>[2x]MNVTVDQSTLAGATRGIVRGGETLKEHRDRLMAATKATGRYAGLKTLELREREPILYNKLFSRLRAGVVDARETAKKIAASPIVEQEGELCFTLYNAAGDSLLTSTGIIIHVGTMGAAIKYMIENNWEANPGVHDKDIFCNNDSLIGNVHPCDIHTIVPIFWEGELIGWVGGVTHVIDTGAVGPGSMATGQVQRFGDGYSITCRKVGANDTLFRDWLHESQRMVRTTRYWMLDERTRIAGCHMIRKLVEEVVAEEGIEAYWKFAYEAVEHGRLGLQARIKAMTIPGTYRQVGFVDVPYAHEDVRVPSDFAKLDTIMHAPCEMTIRRDGTWRLDFEGSSRWGWHTYNAHQVSFTSGIWVMMTQTLIPSEMINDGAAYGTEFRLPKGTWMNPDDRRVAFSYSWHFLVSAWTALWRGLSRSYFGRGYLEEVNAGNANTSNWLQGGGFNQYDEIHAVNSFECAANGTGATAVQDGLSHAAAIWNPEGDMGDMEIWELAEPLVYLGRQIKASSGGSGKYRGGCGFESLRMVWNAKDWTMFFMGNGHISSDWGLMGGYPAASGYRFAAHKTNLKELIASGAEIPLGGDTDPENPTWDAMLPDAQIKRDKQAITTEEMFSDYDLYLNYMRGGPGFGDPLDREPQAVADDINGGYVLERFAGEVYGVVVRKGADGQYGVDEAGTAAARAQIRKDRLAKSVPVSEWMKGEREKILAKDAGTQVRQMFAASFKLGPRFEKDFRTFWSLPDSWTLPEEEIGVPTYGSRYSMDISELPDVHTVQFVEE;>MHHHHHHSSGMNVPVGHLRNVQVLGIDAGGTMTDTFFVDQDGDFVVGKAQSTPQNEALGLIASSEDGLANWGMSLHEALAQLQTGVYSGTAMLNRVVQRKGLKCGLIVNRGMEDFHRMGRAVQSHLGYAYEDRIHLNTHRYDPPLVPRHLTRGVVERTDMIGTQVIPLREDTARDAARDLIAADAEGIVISLLHSYKNPENERRVRDIVLEEVEKSGKKIPVFASADYYPVRKETHRTNTTILEGYAAEPSRQTLSKISNAFKERGTKFDFRVMATHGGTISWKAKELARTIVSGPIGGVIGAKYLGEVLGYKNIACSDIGGTSFDVALITQGEMTIKNDPDMARLVLSLPLVAMDSVGAGAGSFIRLDPYTRAIKLGPDSAGYRVGVCWKESGIETVTISDCHMVLGYLNPDNFLGGAVKLDRQRSVDAIKAQIADPLGLSVEDAAAGVIELLDSDLRDYLRSMISGKGYSPASFVCFSYGGAGPVHTYGYTEGLGFEDVIVPAWAAGFSAFGCAAADFEYRYDKSLDINMPTETPDTDKEKAAATLQAAWEELTKNVLEEFKLNGYSADQVTLQPGYRMQYRGQLNDLEIESPLAQAHTAADWDQLTDAFNATYGRVYAASARSPELGYSVTGAIMRGMVPIPKPKIPKEPEEGETPPESAKIGTRKFYRKKRWVDAQLYHMESLRPGNRVMGPAVIESDATTFVVPDGFETWLDGHRLFHLREV[2x];>MAYTRSKIVDLVDGKIDPDTLHQMLSTPKDPERFVTYVEILQERMPWDDKIILPLGPKLFIVQQKVSKKWTVRCECGHDFCDWKDNWKLSARVHVRDTPQKMEEIYPRLMAPTPSWQVIREYFCPECGTLHDVEAPTPWYPVIHDFSPDIEGFYQEWLGLPVPERADA[2x]

ACs contain metal ions but not organic cofactors, and use ATP to activate substrates through phosphorylation. The first structural rationale for acetone carboxylation is presented here, focusing on the 360 kDa (αβγ)2 heterohexameric AC from Xanthobacter autotrophicus in the ligand-free, AMP-bound, and acetate coordinated states. Like many carboxylases, AC is a heteromultimeric enzyme complex. Its architecture consists of two heterotrimeric αβγ subunits joined by the interacting α-subunits to form a dimeric core.

The AMP-bound structure exhibits dramatic rearrangements of the β-subunits relative to the ligand-free state, with a Cα RMSD difference of 6.3 Å, while the α- and γ-subunits remain almost the same with Cα RMSD of 1.3 Å and 0.3 Å, respectively. First, in the AMP-bound enzyme, the displacement (11–18 Å) of several amino acid residues that participate in nucleotide interactions leads to closing of the substrate-access channel. Most notably, β-Phe405 is displaced by 16 Å, to a new position where it interacts with the adenine of AMP through π-stacking, capping off the access channel. β-Ser391 and the helix of which it is a part rotate into hydrogen bonding distance with the ribosyl moiety. Second, a new internal channel opens up in the AMP-bound structure, connecting the nucleotide-binding site and the Mn site where acetone carboxylation occurs. After nucleotide binding, conformational changes within the β subunit result in loss of an interaction between the side chains of β-Asn578 and α-Glu85 and formation of a new one between β-Asn578 and the carbonyl of β-Met571. The Mn-proximal α-helix concurrently forms a disordered loop (α-81–87), allowing the opening of the substrate channel and the bidentate coordination of the α-Glu89 carboxylate to Mn. The Mn in this structure appears to be coordinately saturated, with α-His150 and α-His175 as monodentate ligands and two side chains each bound in a bidentate mode (α-Asp153, α-Glu89). The structure of AC in the presence of bound AMP and in the absence of these phosphorylated intermediates may therefore represent a trapped state, bound to the product AMP but lacking intermediates needed to proceed further in the reaction. This trapped state reveals the internal channel that is proposed to protect the semistable phosphorylated intermediates from the bulk solvent as they travel from the nucleotide-binding site to the Mn site.> MAYPDANLLNDRVLRAMLKAEETCAPSVSYFKCVQK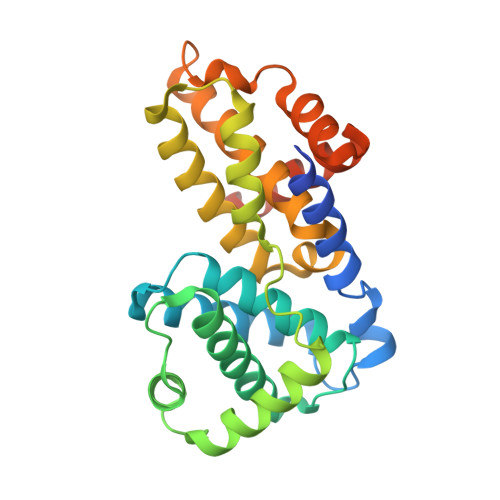EVLPSMRKIVATWMLEVCEEQKCEEEVFPLAMNYLDRFLSLEPVKKSRLQLLGATCMFVASKMKETIPLTAEKLCIYTDNSIRPEELLQMELLLVNKLKWNLAAMTPHDFIEHFLSKMPEAEENKQIIRKHAQTFVALCATDVKFISNPPSMVAAGSVVAAVQGLNLRSPNNFLSYYRLTRFLSRVIKCDPDCLRACQEQIEALLESSLRQAQQNMDPKAA>TYVIAEPCVDVKDKACIEECPVDCIYEGARMLYIHPDECVDCGACEPVCPVEAIYYEDDVPDQWSSYAQANADFFAELGSPGGASK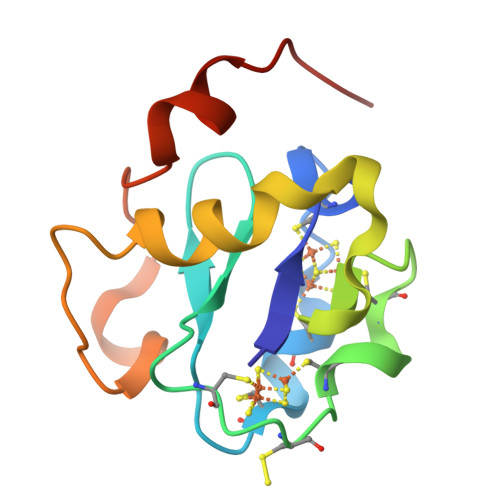VGQTDNDPQAIKDLPPQGE[2x]Norovirus (NoV) is a non-enveloped, positive-stranded RNA virus belonging to the Caliciviridae family. The common capsid structure of 180 copies of the VP1 capsid protein forming a T = 3 icosahedral particle is shared by all identified caliciviruses, which was first reported with HNoV GI.1 virus-like particle (VLP) produced by a baculovirus expression system in 1999. The VP1 protein consists of a shell (S) and protruding (P) domain. Here, using cryo-electron microscopy (cryo-EM), we show that the P domain of MNoV infectious particles reversibly rotates ~70°, in response to aqueous conditions, taking two different conformations; the rising and resting P domain conformations.

Therefore, the VLP of MNoV-S7 was used for the high resolution cryo-EM analysis, and the 3D model was determined at 3.5 Å resolution. Atomic models of the MNoV-S7 VLP capsid were built for the quasi-equivalent A, B, and C monomers of VP1, respectively. For modeling VP1’s A and B monomers, 513 amino acids from Gln19 to Gly531 and 516 amino acids from Ala16 to Gly531 were used, respectively. For modeling VP1’s C monomers, 502 amino acids from Val30 to Gly531 were used. The models were also fitted to the 5.2 and 5.3 Å resolution cryo-EM maps of the MNoV-S7 and MNoV-1 infectious particles with high cross-correlation coefficients of 0.92 and 0.91, respectively, indicating that the structure of MNoV-S7 VLP is highly similar to both the MNoV-S7 and MNoV-1 infectious particles. To understand the capsid structure of the resting P domain conformation, which shows higher levels of infectivity, we investigated the molecular interactions between the P domain dimers of the MNoV-S7 VLP suspended in DMEM. The cryo-EM map of the MNoV-S7 VLP in DMEM revealed several hydrophobic and polar interactions between the neighboring A/B and C/C dimers at the P2 level (yellow in Fig 4). We propose the following chemical interactions between residues on the P domain surface: Asn409, Gly411, Leu412, and Pro415 located on the βF''–βB' loop of the C/C dimer interact with Gln371, Arg373, Val368, and Pro319 located on the βB''–βC'' and βD''–βE'' loops of the A/B dimers, respectively. A new feature found in the structure of MNoV is that the N-terminal arm (NTA) in the A monomer extends to the adjacent A monomer, forming a complex of the fivefold axis. On the other hand, the NTA in the B monomer extends to the adjacent C monomer, forming a complex of the threefold axis, though the NTA in C monomer is more disordered. As a candidate, we found a potential interaction via a metal ion between two carboxylates (Glu223 and Asp231) observed in the folded, flexible hinge of the resting conformation.

>MRMSDGAAPKANGSEASGQDLVPTAVEQAVPIQPVAGAALAAPAAGQINQIDPWIFQNFVQCPLGEFSISPRNTPGEILFDLALGPGLNPYLAHLSAMYTGWVGNMEVQLVLAGNAFTAGKVVVALVPPYFPKGSLTTAQITCFPHVMCDVRTLEPIQLPLLDVRRVLWHATQDQEESMRLVCMLYTPLRTNSPGDESFVVSGRLLSKPAADFNFVYLTPPIERTIYRMVDLPVLQPRLCTHARWPAPIYGLLVDPSLPSNPQWQNGRVHVDGTLLGTTPVSGSWVSCFAAEAAYEFQSGIGEVATFTLIEQDGSAYVPGDRAAPLGYPDFSGQLEIEVQTETTKKGEKLKVTTFEMILGPTTNVDQVPYQGRVYASLTAAASLDLVDGRVRAVPRSVYGFQDVVPEYNDGLLVPLAPPIGPFLPGEVLLRFRTYMRQIDSTDAAAEAIDCALPQEFVSWFASNAFTVQSEALLLRYRNTLTGQLLFECKLYSEGYIALSYSGSGPLTFPTDGFFEVVSWVPRLYQLASVGSLATGRTLKQ[3x]> ATAYTLNLANPSASQYSSFLDQIRNNVRDTSLIYGGTDVEVIGAPSTTDKFLRLNFQGPR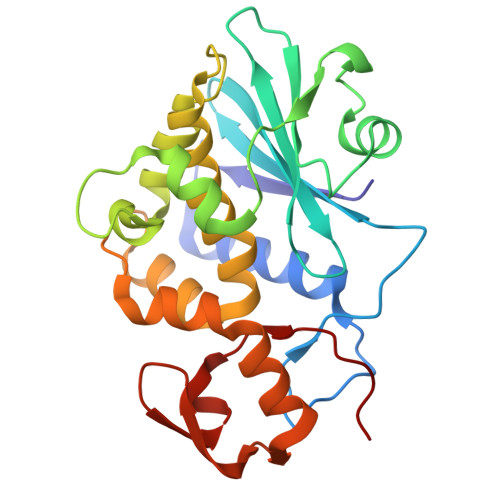GTVSLGLRRENLYVVAYLAMDNANVNRAYYFKNQITSAELTALFPEVVVANQKQLEYGEDYQAIEKNAKITTGDQSRKELGLGINLLITMIDGVNKKVRVVKDEARFLLIAIQMTAEAARFRYIQNLVTKNFPNKFDSENKVIQFQVSWSKISTAIFGDCKNGVFNKDYDFGFGKVRQAKDLQMGLLKYLGRPK>MAHHHHHHMNTIKQDYIEKANALSLSNELNQDQKDLILSIIDKFEDNDPALHNVYQLMIKRVKLGFVFDIAPSVNASEIALFKKDEKLSFNNDNNKPTNTLIIGENYDALKNLIVIESQSETVNYDVIYIDPPYNTESSLSDGNNLSEKDDVGSSKFIYRGKFSRTGWLNMLNERLRMAKQLLKEDGVIF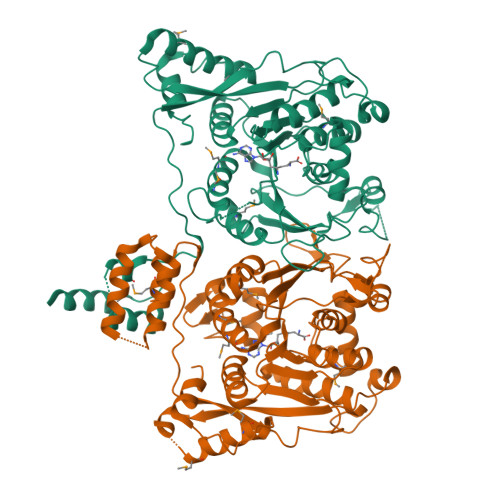VSIDDSEQAYLKVLMDEIFGEENFIACVPAILNPSGRQVNTEIALTHEYILIYGGVNFVPEELDNEYVINKLPEIYKNRNLETLVDNKGEYWLQYTLENQSKKFNDKNRPNLAYPIFINKDENHNLYHTIEPTEKTIYTLWPKNVNGVQYVWRWSREKINKEKEELVIKMDNDKFKIYPKKRKNTWIFKTIIKGSSFNNKTGNKVLSSILKSDEFSTAKPVELIKLLIKLHPNNNARILDFYAGSGTTGHAVMELNKEDGGNRCYTLVTNNENNIATNVCYERLYRINNGIYTNNESNFDWIKKNKPYKSNLNVYDIEYFSTKLFDDNQSNMSIKEQYIKMLQDFNIDTEDKDSNIDILRSLTSLKPISKEDTDAIK[2x]> MAHHHHHHMTSPLRNDRLLRALRREPVDCTPVWLMRQAGRYLPEYRATRAKAGSFLAMAKNPEIACEVTLQPLRRFPLDAAILFSDILTIPDAMGLELYFVEGEGPKFRHPVRDEAAIARLAVPDMEQDLGYVMDAVRLIRRELDGQVPLIGFSGSPWTLACYMVEGGGSKDFARIKAMALNHPQALHRLLEVTTDAVIAYLGAQRAAGAQALQVFDTWGGVLSPAMYREFSLRYLQRIAEGLERGEGSERTPLILFGKGTGLHLEALSQTGADALGLDWTLDLDEA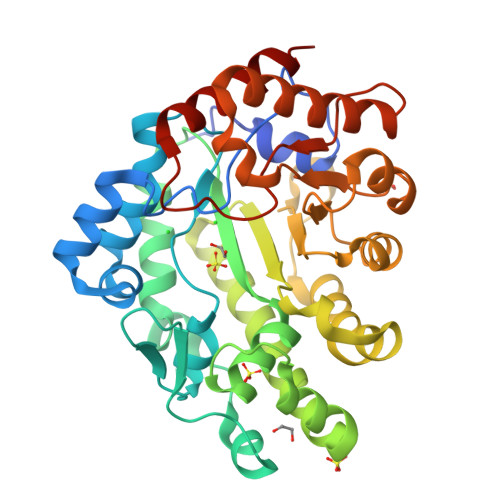MRRTGGRVALQGNLDPTTLYASPDAIAAAAARVLDTYAAGNGGSREGHVFNLGHGMSPDMDPAHVQVLVDAVHAHSQR>[4x]GHMEKRFYILTIVVEDREKAYRQVNEL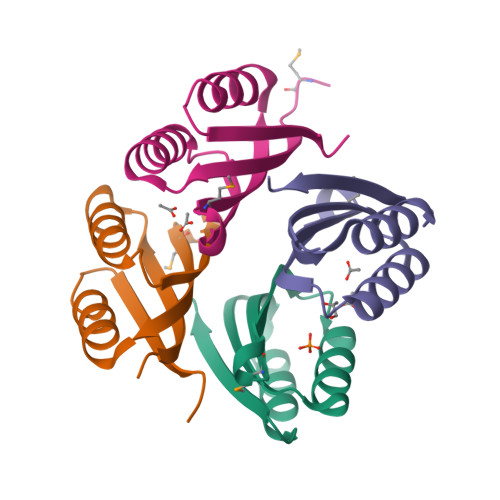LHNFSEDILLRVGYPVREENMAIIFLVLKTDNDTIGALSGKLGQISGVRVKTVPLKRGS>[4x]TWLPLNPIPLKDRVSMIFLQYGQIDVIDGAFVLIDKTGIRTHIPVGSVACIMLEPGTRVSHAAVRLAAQVGTLLVWVGEAGVRVYASGQPGGARSDKLLYQAKLA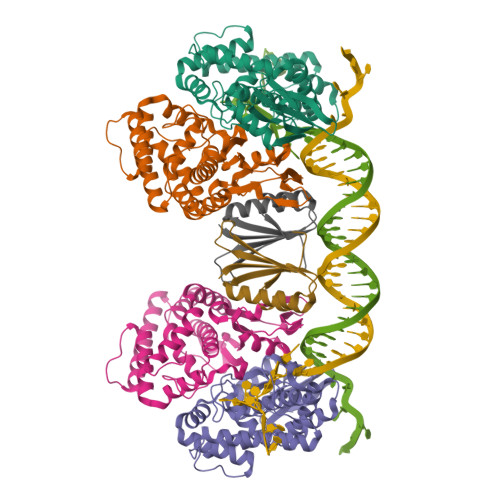LDEDLRLKVVRKMFELRFGEPAPARRSVEQLRGIEGSRVRATYALLAKQYGVTWNGRRYDPKDWEKGDTINQCISAATSCLYGVTEAAILAAGYAPAIGFVHTGKPLSFVYDIADIIKFDTVVPKAFEIARRNPGEPDREVRLACRDIFRSSKTLAKLIPLIEDVLAAGEIQPPA;>[2x]MSMLVVVTENVPPRLRGRLAIWLLEVRAGVYVGDVSAKIREMIWEQIAGLAEEGNVVMAWATNTETGFEFQTFGLNRR> MLRRTVTSLRNARELHRLLPALLPLLDPPVPTGASVCAAHLIVATGHVSKQREPHMSNCPVLERKIPLSEIASDDNFLKHPCVPCLKHRINFLASEDFCYDFVERCGCGTDGALPPEWRCIVERQFGSMAALVEELVIHASNRREAGWTWLV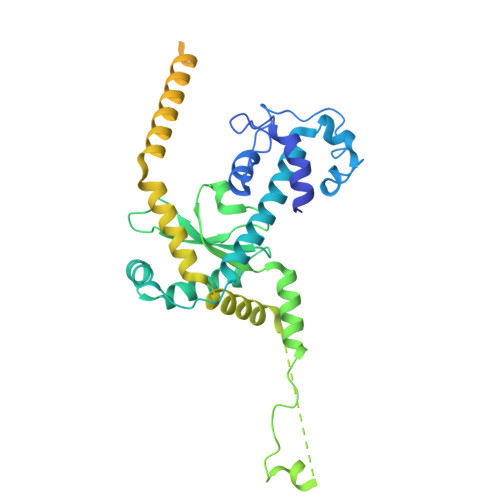YDAQQAGERPLLVVNMPAQRSPLLLGLWPLAVVNVTEAVLVEAVRAESSGSVAAAPPPPWCRAARASLYDTKAAAEAFAMTAPMSEGVGKKLSEIREKVARDAVSRMNWGFILQQLKKAETYYASSDRGEKIRVHRMKLEREAVTKAMSGLRDSGATFLTHDTVEVTTTPSANSEPSSPERVPGVQAKQPQTEGMDPCKNKASAEPDPKCTQLPDGTWQYSYRNGDVTLLKPDGTRVFRKRELTTTAYPDGSMLFQYANNTSILDRADGVRVTTFEDGTTKEEMIRR The potent neurotoxic venom of the black widow spider contains a cocktail of seven phylum-specific latrotoxins (LTXs), but only one, α-LTX, targets vertebrates. This 130 kDa toxin binds to receptors at presynaptic nerve terminals and triggers a massive release of neurotransmitters. Each monomer is composed of an N-terminal four-helix connector domain (CD; residues E21–D115), a central helical bundle domain (HBD; residues S116–K350), a short β-sheet plug domain (PD; residues Q351–D453) and a C-terminal tail of 22 ARs (ARD; residues I454–G1195).

In the second state, the HBDs are moved closer together, forming tight interactions that result in the narrow conformation of the central core. The CD assumes a dramatically different conformation and is completely folded out of its pocket. The four N-terminal CDs are remodeled in an extended coiled-coil needle, whereas the C-terminal domains preserve their overall arrangement. The distal end of the tetrameric coiled-coil needle is formed by the most N-terminal region of the protein (helices α1–α3 in state 1) and might correspond to the transmembrane region of the pore. This domain however is flexible and not resolved in the cryo-EM structure, as might be expected in the absence of a lipid environment or detergents. The particles show characteristic mushroom-like structures resembling the cryo-EM structure of state 2 with the (N-terminal) tip of their needle inserted into the membrane. We, therefore, conclude that the mushroom-like cryo-EM structure of state 2 indeed represents the pore state of α-LTX. During prepore to pore transition, helix α5 separates from the HBD and undergoes a reorientation of almost 180 degrees. This way, it forms an intriguing rigid tetrameric coiled-coil with the α5 helices of the other three monomers. In addition, helix α4 of the CD folds into a continuous helix with α5. In this manner, the coiled-coil elongates, positioning the N-terminal helices α1–α3 of the CD at its lower end to form the transmembrane domain (TMD).

>[4x]EGEDLTLEEKAEICSELELQQKYVDIASNIIGDLSSLPIAGKIAGTIAAAAMTATHVASGRLDIEQTLLGCSDLPFDQIKEVLENRFNEIDRKLDSHSAALEEITKLVEKSISVVEKTRKQMNKRFDEVMKSIQDAKVSPIISKINNFARYFDTEKERIRGLKLNDYILKLEEPNGILLHFKESRTPTDDSLQAPLFSIIEEGYAVPKSIDDELAFKVLYALLYGTQTYVSVMFFLLEQYSFLANHYYEKGYLEKYDEYFNSLNNVFLDFKSSLVGTGTSNNEGLLDRVLQVLMTVKNSEFLGLEKNGVDEMLNEKINLFNKIKEEIEGKQKMTLSETPENFAQISFDKDITTPIGDWRDGREVRYAVQYASETLFSKISHWSDPVSVREKACPTLRMPVDQTRRNVLVFRKFDSSKPQLVGEITPYLSNFIDIDRDLYNAASNPDSAVGFKEFTKLNYDGANIRATFDHGRTVFHAAAKSGNDKIMFGLTFLAKSTELNQPDKKGYTPIHVAADSGNAGIVNLLIQRGVSINSKTYHFLQTPLHLAAQRGFVTTFQRLMESPEININERDKDGFTPLHYAIRGGERILEAFLNQISIDVNAKSNTGLTPFHLAIIKNDWPVASTLLGSKKVDINAVDENNITALHYAAILGYLETTKQLINLKEINANVVSSPGLLSALHYAILYKHDDVASFLMRSSNVNVNLKALGGITPLHLAVIQGRKQILSLMFDIGVNIEQKTDEKYTPLHLAAMSKYPELIQILLDQGSNFEAKTNSGATPLHLATFKGKSQAALILLNNEVNWRDTDENGQMPIHGAAMTGLLDVAQAIISIDATVVDIEDKNSDTPLNLAAQNSHIDVIKYFIDQGADINTRNKKGLAPLLAFSKKGNLDMVKYLFDKNANVYIADNDGMNFFYYAVQNGHLNIVKYAMSEKDKFEWSNTDNNRRDECPNEECAISHFAVCDAVQFDRIEIVKYFVGTLGNFAICGPLHQAARYGHLDIVKYLVEEEFLSVDGSKTDTPLCYASENGHFTVVQYLVSNGAKVNHDCGNGMTAIDKAITKNHLQVVQFLAANGVDFRRKNSRGTTPFLTAVAENALHIAEYLIREKRQDININEQNVDKDTALHLAVYYKNLQMIKLLIKYGIDVTIRNAYDKTALDIAIDAKFSNIVEYLKTKSG Sulfurtransferases, also known as rhodaneses, facilitate the transfer of sulfur from a donor molecule to a thiophilic acceptor. FrST exists as a dimer and can be classified as a TST rather than an MST according to sequence-based clustering and enzyme activity. Each subunit of FrST comprised 11 α-helices, two 310 helices, and six β-strands and was divided into two distinct domains: the N-terminal rhodanese fold domain (non-active domain) and the C-terminal rhodanese fold domain (active domain). The active site of FrST was composed of Trp102, Val176, Arg177, Glu181, Trp211, Arg248, and Arg252, which surrounded catalytic Cys247.

During the crystal structure determination, we also solved another crystal structure of FrST, which belongs to the I21 space group and is annotated as FrSTI21. The overall structure of both structures is almost identical, evidenced by an RMSD of 0.284 Å (Cα). However, when FrSTI21 could closely resemble FrSTP1, a distinct conformational difference was observed in the 8α-η2 loop region at the top of the active site. In contrast, in FrSTI21, Tyr192 tilted toward the active site and engaged in cation π-interaction with Arg252 as well as a hydrogen bond with Glu42. This arrangement resulted in the formation of a cavity for substrate binding, unlike that in FrSTP1. The swinging motion of Tyr192 induced changes in the active site cavity volume of FrST. Volume analysis using ParKVFinder 3.0 revealed that the volume of the active site in FrSTP1was 8.2 Å3, whereas it was 12.3 Å3 in FrSTI21. Three substrates, namely benzenethiosulfonate, methanethiosulfonate, and thiosulfate, were docked at the active site of FrSTI21. The tetrahedral sulfonate or sulfide of each substrate was positioned at the active site in a similar conformation and interacted with the side chains of Glu181 and Arg248 as well as the backbend of Ser178 via hydrogen bonds. The benzene ring of benzenethiosulfonate was located between Tyr192 and Trp211 within a possible range of hydrophobic interactions.

> GSHMSVDLDPSARFAEYAHPERLVSTEWLAAHLGDEGLVVVESDEDVLLYETGHIPGAVKVDWHTDLNDPVQRDYIDGAAFAALLGERGISRDTTVVIYGDKNNWWAAYALWVFTLFGHDDVRLLDGGRSKWEAEGRAYTTDAPTVAATSYPVVERDDSRIRAYRDDVLAHFGKPLIDVRSPEEFSGARTTAPAYPEEGALRAGHIPSAQNVPWGKAAAEDGTFRTLAELDALYRDGAGLKDGDDVVAYCRIGERSSHTWFVLQHLLGFENVRNYDGSWTEWGSAVRVPIVQGSEPGEAPAPIVGR> GGG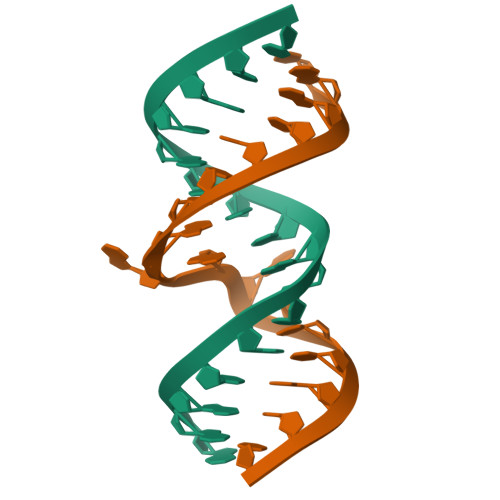CGUCGCUAGUACC;> CGGUACUAAAAGUCGCC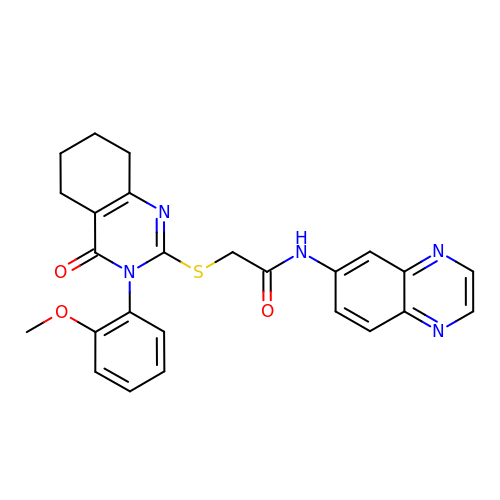2-{[3-(2-METHOXYPHENYL)-4-OXO-3,4,5,6,7,8-HEXAHYDROQUINAZOLIN-2-YL]SULFANYL}-N-QUINOXALIN-6-YLACETAMIDE | C25 H23 N5 O3 S | AXVDURNCPXUGDZ-UHFFFAOYSA-N> GLDRNRQDIGYVLGRLFAVLEKIQAEANPGLNATIADRYFGSASSTPIAVFGTLMRLLPHHLNKLEFEGRAVQLQWEIRQILEHCQRFPNHLNLEQQGLFAIGYYHETQFLFTKDALKNLFNE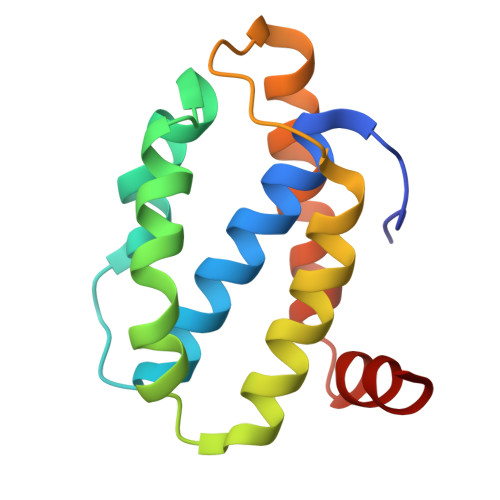A>[2x]GSHMRKQQRMVVVRAEGGGGINPEIRKNEDKVVDSVVVTELSKNITP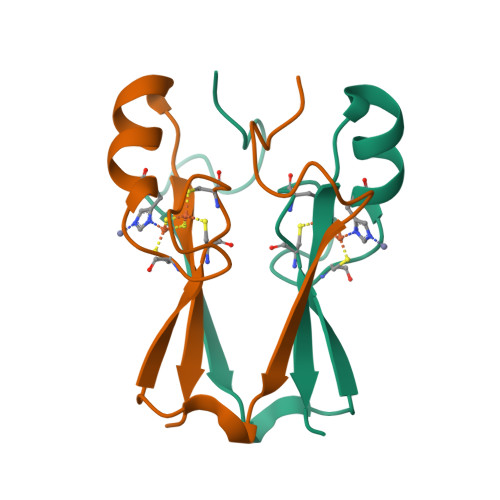YCRCWRSGTFPLCDGSHVKHNKANGDNVGPLLLKKQ8-(3-methyl-1-benzofuran-5-yl)-~{N}-(4-methylsulfonylpyridin-3-yl)quinoxalin-6-amine 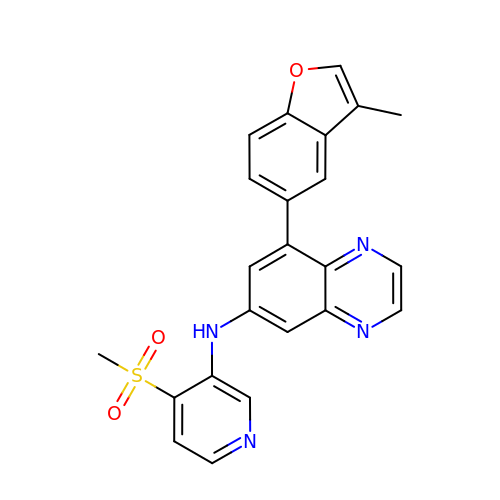| C23 H18 N4 O3 S | OTFZEDIHBPYVKA-UHFFFAOYSA-N>[4x]GMTIYTLSHGSLKLDVSDQ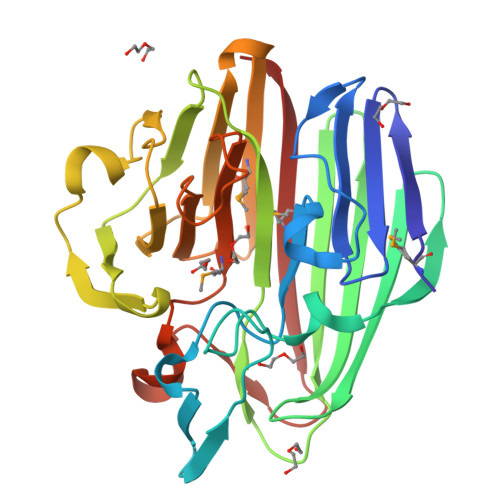GGVIEGFWRDTTPLLRPGKKSGVATDASCFPLVPFANRVSGNRFVWQGREYQLQPNVEWDAHYLHGDGWLGEWQCVSHSDDSLCLVYEHRSGVYHYRVSQAFHLTADTLTVTLSVTNQGAETLPFGTGWHPYFPLSPQTRIQAQASGYWLEREQWLAGEFCEQLPQELDFNQPAPLPRQWVNNGFAGWNGQARIEQPQEGYAIIMETTPPAPCYFIFVSDPAFDKGYAFDFFCLEPMSHAPDDHHRPEGGDLIALAPGESTTSEMSLRVEWL[[[[(2R,5S)-5-(4-azanyl-2-oxidanylidene-pyrimidin-1-yl)-1,3-oxathiolan-2-yl]methoxy-oxidanyl-phosphoryl]oxy-oxidanyl-phosphoryl]amino]phosphonic 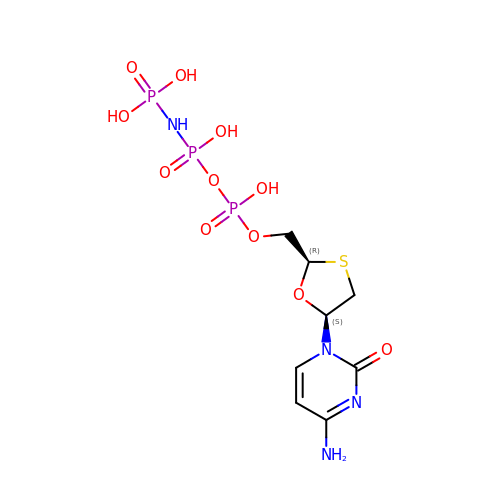acid | C8 H15 N4 O11 P3 S | KGYPGPIERPVYLF-NKWVEPMBSA-N>MKNTGDEVVAIISQNGKVIREIPLTGHKGNEQFTIKGKGAQYNLMEVDGERIRIKEDNSPDQVGVKMGWKSKAGDTIVCLPHKVFVE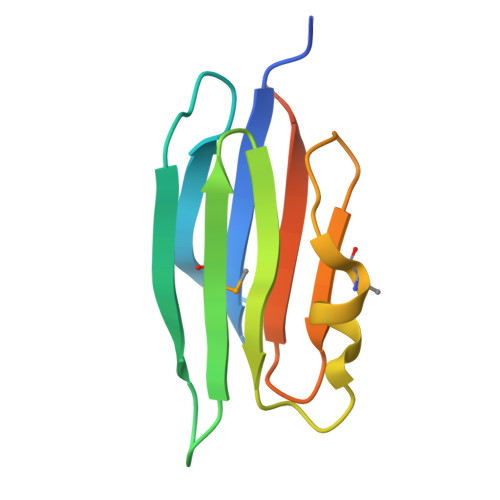IKSTQKLEHHHHHH[3x]> MANTRYK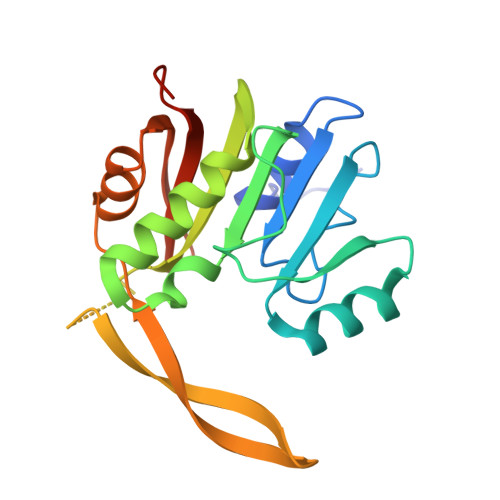PWPIVEKFLRDQKDHSVGVDIGCGNGKYMGVNNKVFIVGSDRSDELVKLAHDMDPSREVVVCDAIDNAHPEGRFDFAISIAVIHHFSTPERRREAVRAILNTLRPDGRALIYVWALEQKTSRRGWHEGMDQDVMVPWVKKVDGVEEVRYRYYHLYREGEITSDVEASGGKVLETGYEKDNWWVVAKRGDDWSHHHHHH> MQVNRLPFFTNHFFDEYLLISEDTPVGSSVTQLLARDMDNDPLVFGVSGEEASRFFAVEPDTGVVWLRQPLDRETKSEFTVEFSVSDHQGVITRKVNIQVGD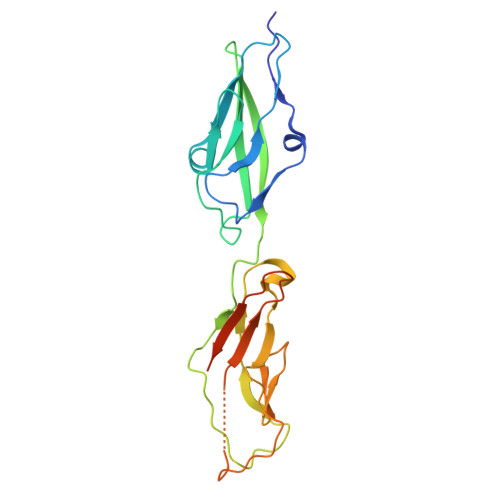VNDNAPTFHNQPYSVRIPENTPVGTPIFIVNATDPDLGAGGSVLYSFQPPSPFFAIDSARGIVTVIQELDYEVTQAYQLTVNATDQDKTRPLSTLANLAIIITDLEHHHHHH Herein, we describe the biochemical and structural characterization of two multi-FMN-containing covalent flavoproteins, SaFMN3 from Streptomyces azureus and CbFMN4 from Clostridiaceae bacterium. Based on their primary structure, these proteins were predicted to contain three and four covalently tethered FMN cofactors, respectively. Recently, Méheust et al. discovered by sequence analysis a multitude of sequences of extracytosolic proteins predicted to contain multiple covalently bound FMN molecules. Such multi-FMN binding proteins are thought to play a role in extracellular long-distance electron transfer paths similar to multi-heme proteins. The crystal structures were elucidated, which confirmed that the flavin cofactor is covalently attached to a threonine.

The asymmetric unit of the CbFMN4-D1 crystal contains two protein molecules. The CbFMN4-D1 structure consists, like SaFMN3-D2, of an anti-parallel sheet (residues 1–9, 14–22, and 25–33) and two α-helices (residues 38–56 and 67–83). Hydrogen bonds are observed between the N-terminal strands of the two molecules. The dimer interface appears to have resulted from crystal packing. Tyr11 stacks on one site of the isoalloxazine (analogous to Tyr14 in SaFMN3-D2), while Leu40 is situated on the other site (analogous to Ile45 in SaFMN3-D2). Additionally, mostly analogous hydrogen bonds are observed between the O2 of FMN and the backbone amides of Val68 and Ser69, the N3 with Ser69-Oγ1, the O4 with the backbone amide of Thr37, and N5 with the Oγ1 of Thr37, while the O4’ of the ribityl group has a hydrogen bond with the backbone amide of Thr67. Both CbFMN4-D1 molecules have a covalently bound FMN via Thr67. The structure of CbFMN4-D1 is similar to SaFMN3-D2 (their Cα r.m.s.d is 1.7 Å) while there is only 18% sequence identity. The highest similarity is observed in the FMN binding sequence motif. Structural elucidation of a domain of this flavoprotein revealed a similar overall structure and binding mode of the FMN cofactor.

>[2x]MLSYEVTAEGYGGPIRLMVYVEGEEIVDIEVLEENETPNLGDVAIEEMITKILEGQSTDVDVHSGATVSSNAVIEAVKQAMAEAG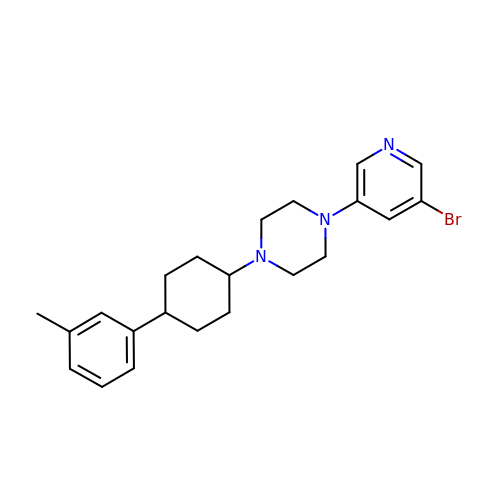1-(5-bromopyridin-3-yl)-4-[cis-4-(3-methylphenyl)cyclohexyl]piperazine | C22 H28 Br N3 | GPGOZHVXQXMXPF-RVWIWJKTSA-N>[4x]MSEMSSFLHIGDIVSLYAEGSVNGFISTLGLVDDRCVVEPAAGDLDNPPKKFRDCLFKVCPMNRYSAQKQYWKAKQTKQDKEKIADVVLLQKLQHAAQMEQKQNDTENKKVHGDVVKYGSVIQLLHMKSNKYLTVNKRLPALLEKNAMRVTLDATGNEGSWLFIQPFWKLRSNGDNVVVGDKVILNPVNAGQPLHASNYELSDNAGCKEVNSVNCNTSWKINLFMQFRDHLEEVLKGGDVVRLFHAEQEKFLTCDEYKGKLQVFLRTTLRQSATSATSSNALWEVEVVHHDPCRGGAGHWNGLYRFKHLATGNYLAAEENPSYKGDASDPKAAGMGAQGRTGRRNAGEKIKYCLVAVPHGNDIASLFELDPTTLQKTDSFVPRNSYVRLRHLCTNTWIQSTNVPIDIEEERPIRLMLGTCPTKEDKEAFAIVSVPVSEIRDLDFANDASSMLASAVEKLNEGFISQNDRRFVIQLLEDLVFFVSDVPNNGQNVLDIMVTKPNRERQKLMREQNILKQVFGILKAPFREKGGEGPLVRLEELSDQKNAPYQHMFRLCYRVLRHSQEDYRKNQEHIAKQFGMMQSQIGYDILAEDTITALLHNNRKLLEKHITKTEVETFVSLVRKNREPRFLDYLSDLCVSNHIAIPVTQELICKCVLDPKNSDILIRTELRPVKEMAQSHEYLSIEYSEEEVWLTWTDKNNEHHEKSVRQLAQEARAGNAHDENVLSYYRYQLKLFARMCLDRQYLAIDEISQQLGVDLIFLCMADEMLPFDLRASFCHLMLHVHVDRDPQELVTPVKFARLWTEIPTAITIKDYDSNLNASRDDKKNKFANTMEFVEDYLNNVVSEAVPFANEEKNKLTFEVVSLAHNLIYFGFYSFSELLRLTRTLLGIIDCVQGPPAMLQAYEDPGGKNVRRSIQGVGHMMSTMVLSRKQSVFSAPSLSAGASAAEPLDRSKFEENEDIVVMETKLKILEILQFILNVR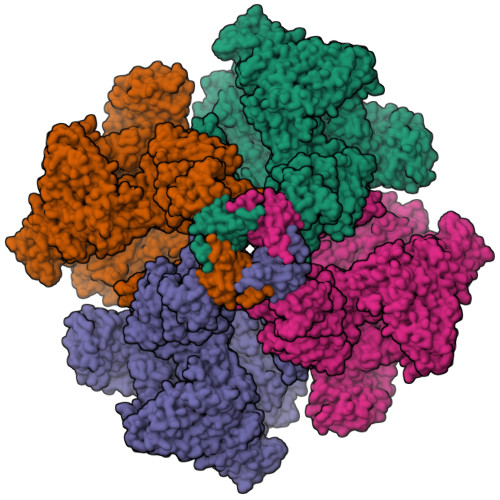LDYRISYLLSVFKKEFVEVFPMQDSGADGTAPAFDSTTANMNLDRIGEQAEAMFGVGKTSSMLEVDDEGGRMFLRVLIHLTMHDYAPLVSGALQLLFKHFSQRQEAMHTFKQVQLLISAQDVENYKVIKSELDRLRTMVEKSELWVDKKGSGKGEEVEAGAAKDKKERPTDEEGFLHPPGEKSSENYQIVKGILERLNKMCGVGEQMRKKQQRLLKNMDAHKVMLDLLQIPYDKGDAKMMEILRYTHQFLQKFCAGNPGNQALLHKHLHLFLTPGLLEAETMQHIFLNNYQLCSEISEPVLQHFVHLLATHGRHVQYLDFLHTVIKAEGKYVKKCQDMIMTELTNAGDDVVVFYNDKASLAHLLDMMKAARDGVEDHSPLMYHISLVDLLAACAEGKNVYTEIKCTSLLPLEDVVSVVTHEDCITEVKMAYVNFVNHCYVDTEVEMKEIYTSNHIWTLFENFTLDMARVCSKREKRVADPTLEKYVLSVVLDTINAFFSSPFSENSTSLQTHQTIVVQLLQSTTRLLECPWLQQQHKGSVEACIRTLAMVAKGRAILLPMDLDAHISSMLSSGASCAAAAQRNASSYKATTRAFPRVTPTANQWDYKNIIEKLQDIITALEERLKPLVQAELSVLVDVLHWPELLFLEGSEAYQRCESGGFLSKLIQHTKDLMESEEKLCIKVLRTLQQMLLKKTKYGDRGNQLRKMLLQNYLQNRKSTSRGDLPDPIGTGLDPDWSAIAATQCRLDKEGATKLVCDLITSTKNEKIFQESIGLAIHLLDGGNTEIQKSFHNLMMSDKKSERFFKVLHDRMKRAQQETKSTVAVNMNDLGSQPHEDREPVDPTTKGRVASFSIPGSSSRYSLGPSLRRGHEVSERVQSSEMGTSVLIMQPILRFLQLLCENHNRDLQNFLRCQNNKTNYNLVCETLQFLDIMCGSTTGGLGLLGLYINEDNVGLVIQTLETLTEYCQGPCHENQTCIVTHESNGIDIITALILNDISPLCKYRMDLVLQLKDNASKLLLALMESRHDSENAERILISLRPQELVDVIKKAYLQEEERENSEVSPREVGHNIYILALQLSRHNKQLQHLLKPVKRIQEEEAEGISSMLSLNNKQLSQMLKSSAPAQEEEEDPLAYYENHTSQIEIVRQDRSMEQIVFPVPGICQFLTEETKHRLFTTTEQDEQGSKVSDFFDQSSFLHNEMEWQRKLRSMPLIYWFSRRMTLWGSISFNLAVFINIIIAFFYPYMEGASTGVLDSPLISLLFWILICFSIAALFTKRYSIRPLIVALILRSIYYLGIGPTLNILGALNLTNKIVFVVSFVGNRGTFIRGYKAMVMDMEFLYHVGYILTSVLGLFAHELFYSILLFDLIYREETLFNVIKSVTRNGRSILLTALLALILVYLFSIVGFLFLKDDFILEVDRLPNNHSTASPLGMPHGAAAFVDTCSGDKMDCVSGLSVPEVLEEDRELDSTERACDTLLMCIVTVMNHGLRNGGGVGDILRKPSKDESLFPARVVYDLLFFFIVIIIVLNLIFGVIIDTFADLRSEKQKKEEILKTTCFICGLERDKFDNKTVSFEEHIKLEHNMWNYLYFIVLVRVKNKTDYTGPESYVAQMIKNKNLDWFPRMRAMSLVXXXXXXXXXXXXXXXXXXXXXX> EDKIMSYNAFFWMWVHDMLIDSIKWRDEHGRCINKDKGKTCIKGCNKKCICFQKWVEQKKTEWGKIKDHFRKQKDIPKDWTHDDFLQTLLMKDLLLEIIQDTYGDANEIKRIEALLEQAGVGGIDFAALAGLYTKGFVAEK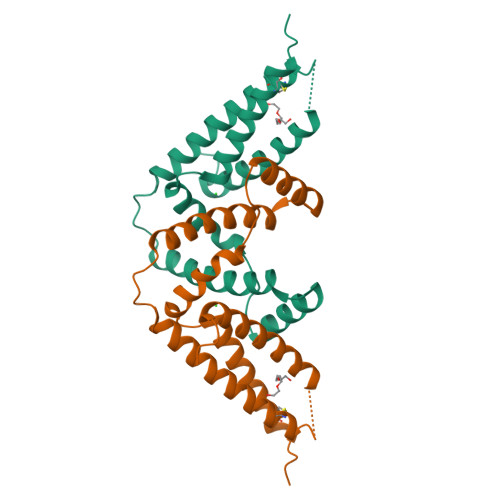DTTIDKLLQHEQKEADKCLKTHTDDTCPPQEDRSVARS>[5x]QDMVSPPPPIADEPLTVNTGIYLIECYSLDDKAETFKVNAFLSLSWKDRRLAFDPVRSGVRVKTYEPEAIWIPEIRFVNVE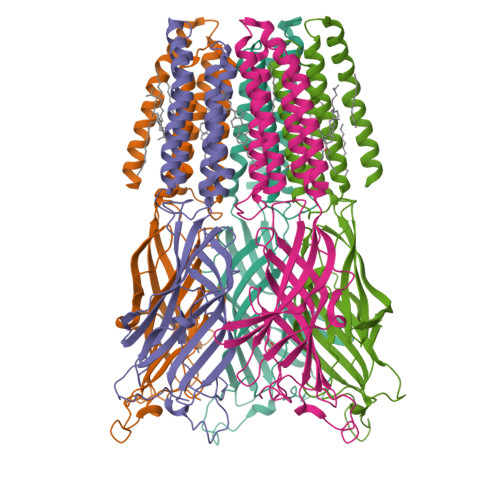NARDADVVDISVSPDGTVQYLERFSARVLSPLDFRRYPFDSQTLHIYLIVRSVDTRNIVLAVDLEKVGKNDDVFLTGWDIESFTAVVKPANFALEDRLESKLDYQLRISRQYGYFVIQTYLPCIMTVILSQVSFWLNRESVPARTVFVVTTVLTMTTLSISARNSLPKVAYATAMDWFIAVCYAFVFSALIEFATVNYFTKSQPARAAKIDRLSRIAFPLLFGIFNLVYWATYLNREPQLKAPTPHQHHHHHHHH5-{3-(S)-(4-(R)-ACETYLAMINO-4-CARBOXY-BUTYRYLAMINO)-3-[1-(R)-(1-(R)-CARBOXY-ETHYLCARBAMOYL)-ETHYLCARBAMOYL]-PROPYL}-2-(CARBOXY-PHENYLACETYLAMINO-METHYL)-3,6-DIHYDRO-2H-[1,3]THIAZINE-4-CARBOXYLIC 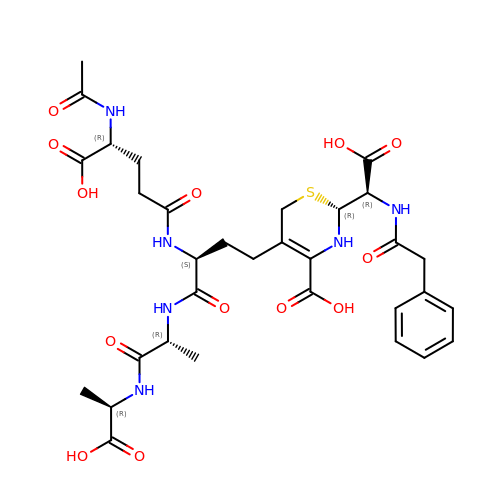ACID | C32 H42 N6 O13 S | PEUIVMLYMKXUBF-PULJXETJSA-N>MLGIVIATHGALSDGAKDAATVIMGATENIETVNL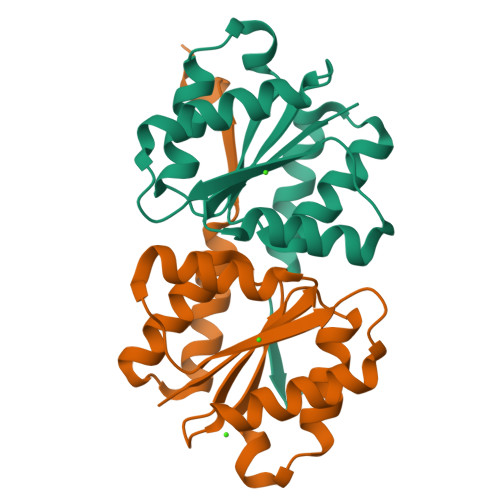NSGDDVQALGGQIKTAIENVQQGDGVLVMVDLLSASPYNQAVLVINELEPALQKKIFVVSGTNLPMVLEAINHQLLGTPIAEAAQAIVAQGKESVQAWDISMTSFEDEEDEDDDF[6x]>KPRKARTAFSDHQLNQLERSFERQKYLS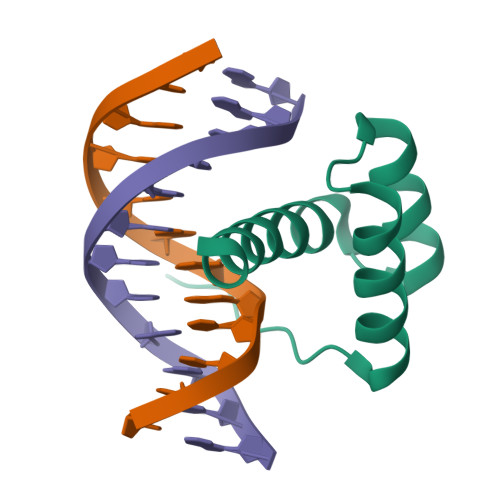VQDRMDLAAALNLTDTQVKTWYQNRRTKWKRQTA[6x]> LQTARKSTGG;> GPLGSPEFMAQGTLIRVTPEQPTHAVCVLGTLTQLDICSSAPEDCTSFSINASPGVVVDIAHSPPAKKKSTGSSTWPLDPGVEVTLTMKAASGSTGDQKVQISYYGPKTPPVKALLYLTAVEISLCADITRTGKVKPTRAVKDQRTWTWGPCGQGAILLVNCDRDNLESSAMDCEDDEVLDSEDLQDMSLMTLSTKTPKDFFTNHTLVLHVARSEMDKVRVFQATRGKLSSKCSVVLGPKWPSHYLMVPGGKHNMDFYVEALAFPDTDFPGLITLTISLLDTSNLELPEAVVFQDSVVFRVAPWIMTPNTQPPQEVYACSIFENEDFLKSVTTLAMKAKCKLTICPEEENMDDQWMQDEMEIGYIQAPHKTLPVVFDSPRNRGLKEFPIKRVMGPDFGYVTRGPQTGGISGLDSFGNLE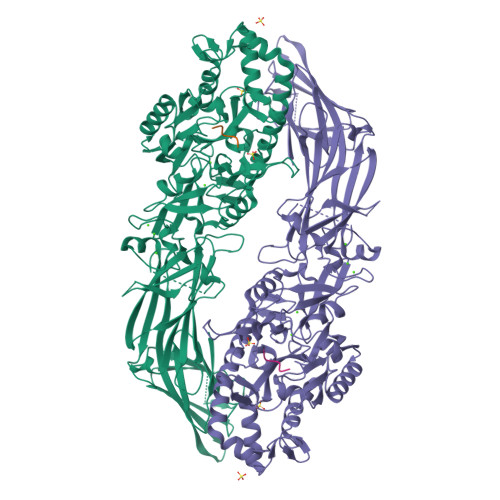VSPPVTVRGKEYPLGRILFGDSCYPSNDSRQMHQALQDFLSAQQVQAPVKLYSDWLSVGHVDEFLSFVPAPDRKGFRLLLASPRSCYKLFQEQQNEGHGEALLFEGIKKKKQQKIKNILSNKTLREHNSFVERCIDWNRELLKRELGLAESDIIDIPQLFKLKEFSKAEAFFPNMVNMLVLGKHLGIPKPFGPVINGRCCLEEKVCSLLEPLGLQCTFINDFFTYHIRHGEVHAGTNVRRKPFSFKWWNMVP>MGSDKIHHHHHHMKAVYPGSFDPITLGHVDI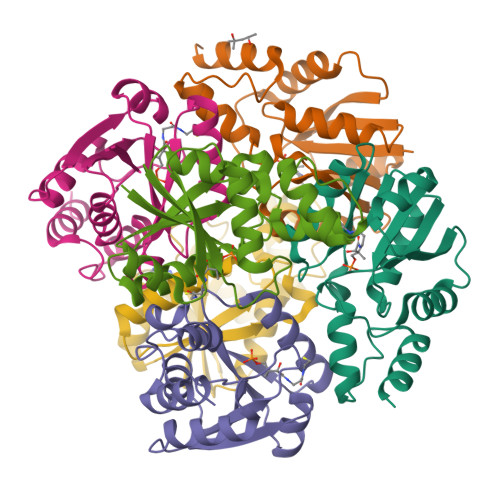IKRALSIFDELVVLVTENPRKKCMFTLEERKKLIEEVLSDLDGVKVDVHHGLLVDYLKKHGIKVLVRGLRAVTDYEYELQMALANKKLYSDLETVFLIASEKFSFISSSLVKEVALYGGDVTEWVPPEVARALNEKLKEGKR[6x]[5-CHLORO-1H-INDOL-2-CARBONYL-PHENYLALANINYL]-AZETIDINE-3-CARBOXYLIC 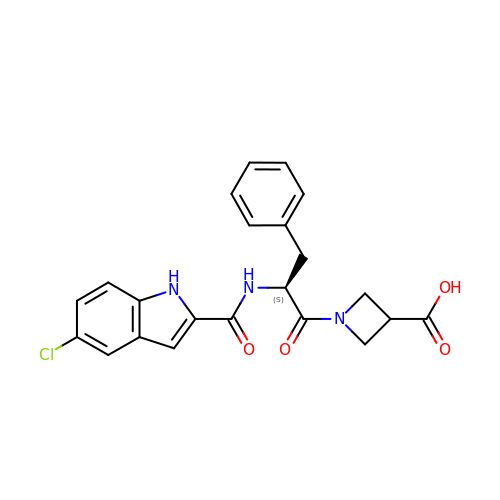ACID | C22 H20 Cl N3 O4 | RONLONYAIBUEKT-IBGZPJMESA-N> MIPINIKDFNYSDPVNNQDIILVKNEKGSFDKGFFVADKILLVPARYGNISTDEGGITSKKEKAHVDKKIYLETDSEKNEYLKNMTTLLKRMNSYSTGNKLLNLIIKGEPIYSKDLQGKFIEQTPSRYLDTNTGKRRVNVMITGPGSNVLTKKCTHNGMGLENDPNGKHSNGTGILSTIEFSPNYLIAYNKCVADPVLTLFHELVHSMHNLYGIAFPDNVKVPYNALKDKNLVSGEEALSEILTFGGKDLTTEHLETLWKKLAETVIIVKDFVKTDTQAKDVFLNNLRFLSKNENIKIDTIEDIVNGTLKIKNNISNLTECEFCKEIGDVRIRTRYAVHSEDVTPVEVVDFKNNYKLNSGFLEGQDISKKYFITNPPKMRRRALRNFKCTIQ;> MADIIASVDKKDVFAVSDTSYFKNFKFPSKKISDTGEVIDSTKLPQIKDTYKSSREEPIPDNDSTINVKNITTYHYLEAQKPKNSSIELTMVAPSKSKKPNDCVVEAINDNNKIYTPFSGTAKQFNTVVPIANTAANVITWLEAIADIFSSETGTFDKLERAGKETLYYIPYVGQLLSIGENVLIGDFKNALLNTGLIILLDIAPELNIPLLGAFEAYKEYKSLEEFRKAIDNVIDERNKRWHSVYSFVAHQWYGQVNIQIEQRLNHFYQALSYQAGVIKNRVDIEYARHKEGLEEKEERKLMWASVDCIGSIEASVKEATKNAEKFLEKSSILYFKEEILPKVHKNLEEFDKNTLFNIYTNIDEFSNRGIAEISECKKVEADVNNGFRPIKFDFSLLTNLMKSDSLTDEVILEKALEDALVFSLGVRNGKIQNLSKKWANLTIGTDIRVVHGRDNESIRLNSTQDSSIQIEKNTNLRFLDSENFSLSFWIRVPRYNKFDKDKDLNNEYTIVNNMDTATKGFKISIKNGILLWTLKGTQQKTIEIPLSNTKVSDNIWRHVAIINNKDGNCTIYVDGAQKNAVSLSGLD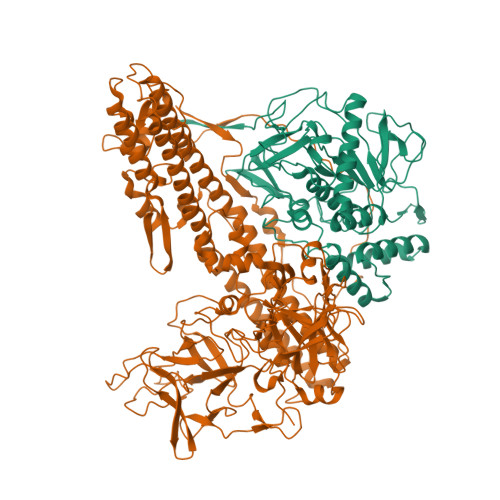EITNTLPITLQLVGNKNKKQFIRLDQFNIYEKALSQTEVGKLFSSYFKDSDIRDYWGEPLAYNKTYNMINIAYQGRGLQSTNNKISLQPKAVFDPTGDGSYIPRLYRGYDVLLQKDSQSKTTDIMPKKDDLINIKLKSGHNFVGFNSTIDTSQKYLKLTTALLSEVDDPKGFKLMSLKKDNWIQIKKETWMSKNGNVIPQGLVGKRSVDSDVYLYLWDWETEKDDYSEKQWSFICQDEGWIDSDGMFTNA One of these oxidoreductases, the metal-containing formate dehydrogenase, catalyses the following redox reaction: 1 CO2+2e−+H+⇌HCOO−,E∘,=−420mV In standard state, the equilibrium of the reaction favours formate oxidation at the active site Mo or W atom, which is energetically coupled to the reduction of oxidised nicotinamide adenine dinucleotide (NAD+) in cytoplasmic FDHs e.g. from Rhodobacter capsulatus and Cupriavidus necator. The RcFDH complex forms a 360 kDa dimer of FdsABGD heterotetramers. Subunit FdsA binds the bis-MGD cofactor, which coordinates the Mo atom in the active site together with the conserved Cys386 residue. The direct electron transfer chain between bis-MGD and FMN of the heterotetramer measures 76 Å and consists of five Fe-S clusters: A1, A2, A3, A5 and B6.

In order to structurally investigate this partially reduced state of the enzyme, we determined the cryo-EM structure of RcFDH in the presence of NADH and azide at 3.2 Å resolution. The atomic model derived from this structure overlays with the coordinates of the as isolated state with a root mean square deviation of 0.31 Å over all but 20 Cα atoms of the four peptide chains. The strong similarity between both structures extends to the active site residues and cofactors, whose location and orientation are indistinguishable between the two states. The difference density between the maps of the NADH reduced and the as isolated enzyme shows a distinct density for NADH near the FMN binding site. Instead of stacking underneath the isoalloxazine ring of FMN, the nicotinamide moiety of NADH sits in front of the FMN binding pocket in hydrogen bond distance to the backbone of FdsB. In this position it blocks access to the binding pocket and also prevents FMN from disengaging from the enzyme, but it is too far away (11.6 Å) to allow for productive electron transfer between NADH and FMN. In contrast, the coordination of the adenosine diphosphate (ADP) moiety of NADH resembles that of complex I. Conserved residues Glu259 and Lys157 form hydrogen bonds to the ribose oxygens of NADH and the alcohol groups of FMN contact the second phosphate group of ADP. More importantly, the negative charge on Glu258 in FdsB repels the phosphate residues of NADH and may contribute to the non-productive positioning of the nicotinamide moiety. Our cryo-EM analysis of two different redox states of RcFDH shows that NADH reduction leads to charging of the cofactors in the absence of the second substrate at the bis-MGD.

>MKDLIIPPLDWTQDMGTPKREGAPVHLTIDGVEVTVPAGTSVLRAAAEAGISIPKLCATDNVEPVGSCRLCMVEIEGMRGTPTSCTTPVAPGMRVHTQTPQLQKLRRGVMELYISDHPLDCLTCAANGDCELQDMAGAVGLREVRYQAKDTHFARRDATGPNPRYIPKDNSNPYFSYDPAKCIVCMRCVRACEEVQGTFALTVMGRGFDARISPAAPDFLSSDCVSCGACVQACPTATLVEKSVERIGTPERKVVTTCAYCGVGCSFEAHMLGDQLVRMVPWKGGAANRGHSCVKGRFAYGYATHQDRILKPMIRDKITDPWREVNWTEALDFTATRLRALRDSHGADALGVITSSRCTNEETYLVQKLARAVFGTNNTDTCARVCHSPTGYGLKQTFGTSAGTQDFDSVEETDLALVIGANPTDGHPVFASRLRKRLRAGAKLIVVDPRRIDLLNTPHRGEAWHLQLKPGTNVAVMTAMAHVIVTEQIFDKRFIGDRCDWDEWADYAEFVANPEYAPEAVESLTGVPAGLLRQAARAYAAAPNAAIYYGLGVTEHSQGSTTVIAIANLAMMTGNIGRPGVGVNPLRGQNNVQGSCDMGSFPHEFPGYRHVSDDATRGLFERTWGVTLSSEPGLRIPNMLDAAVEGRFKALYVQGEDILQSDPDTRHVSAGLAAMDLVIVHDLFLNETANYAHVFLPGSTFLEKDGTFTNAERRINRVRRVMAPKAGFADWEVTQMLANALGAGWHYTHPSEIMAEIAATTPGFAAVTYEMLDARGSVQWPCNEKAPEGSPIMHVEGFVRGKGRFIRTAYLPTDEKTGPRFPLLLTTGRILSQYNVGAQTRRTENTVWHGEDRLEIHPTDAETRGIRDGDWVRLASRAGETTLRATVTDRVSPGVVYTTFHHPDTQANVVTTDTSDWATNCPEYKVTAVQVAASNGPSDWQQDYAAQAAAARRIEAAE[2x];>[2x]MKIWLPCDAAAKACGAEAVLAALRLEAEKRGGALDIARNGSRGMIWLEPLLEVETPAGRIGFGPMTPADVPALFDALESHPKALGLVEEIPFFKRQTRLTFARCGRIEPLSLAQFAAAEGWAGLRKALKMTPAEVVEEVLASGLRGRGGAGFPTGIKWRTVAAAQADQKYIVCNVDEGDSGSFADRMLIEGDPFCLVEGMAIAGHAVGATRGYVYIRSEYPDAIAVMRAAIAMAKPFLAEAGFEMEVRVGAGAYVCGEETSLLNSLEGKRGTVRAKPPLPALKGLFGKPTVVNNLLSLAAVPWIIAHGAKAYESFGMDRSRGTIPLQIGGNVKRGGLFETGFGITLGELVEDICGGTASGRPVKAVQVGGPLGAYHPVSDYHLPFCYEQFAGQGGLVGHAGLVVHDDTADMLKLARFAMEFCAIESCGTCTPCRIGAVRGVEVIDRIAAGDASAMPLLDDLCQTMKLGSLCALGGFTPYPVQSAIRHFPADFPCAREAAE;>[2x]MTDTARLRAILAAHRGREGALLPILHDVQAAFGFIPEDAYAPIAADLGLTRAEVAGVVGFYHDFRKAPAGRHVIKLCRAEACQAMGMDAVQARLESALGLRLGDSSEAVTLEAVYCLGLCACAPAAMVDDRLVGRLDAAAVAGIVAELGA;>MSDDKIIRMANQIAAFFAVQPGDRAGPVAAHISENWSAPMRAALLAHVAAQSPGLDPLVIAAAPQIRPVPA[2x]> GSHMPKMEVFQEYYGIPPPPGAFGPFLRLNPGDIVELTKAEAEHNWWEGR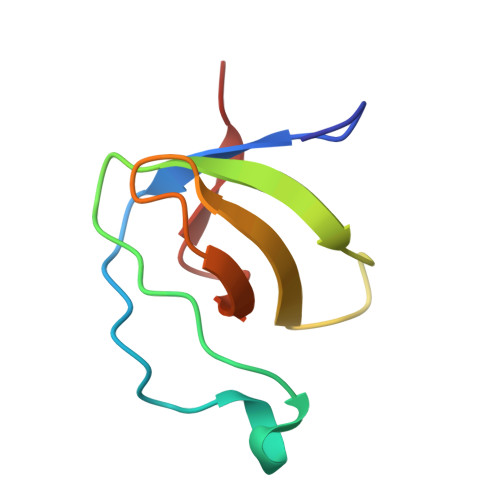NTATNEVGWFPCNRVHPYVH>MAEP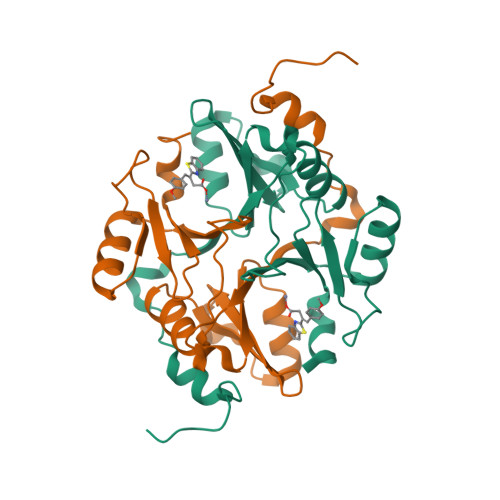QPPSGGLTDEAALSCCSDADPSTKDFLLQQTMLRVKDPKKSLDFYTRVLGMTLIQKCDFPIMKFSLYFLAYEDKNDIPKEKDEKIAWALSRKATLELTHNWGTEDDETQSYHNGNSDPRGFGHIGIAVPDVYSACKRFEELGVKFVKKPDDGKMKGLAFIQDPDGYWIEILNPNKMATLM[2x]> KIPEHLIGKGAEADIKRDSYLDFDVIIKERVKKGYRDERLDENIRKSRTAREARYLALVKDFGIPAPYIFDVDLDNKRIMMSYINGKLAKDVIEDNLDIAYKIGEIVGKLHKNDVIHNDLTTSNFIFDKDLYIIDFGLGKISNLDRDKAVDLIVFKKAVLSTHHEKFDEIWERFLEGYKSVYDRWEIILELMKDVERRARYVE;> MDPMIIRGIRGARINNEIFNLGLKFQILNADVVATKKHVLHAINQAKTKKPIAKSFWMEILVRASGQRQIHEAIKIIGAKDGNVCLICEDEETFRKIYELIGGEIDDSVLEINEDKERLIREIFKIRGFGNVVERVLEKIALIELKKE;> MDPMICLGLEGTAEKTGVGIVTSDGEVLFNKTIMYKPPKQGINPREAADHHAETFPKLIKEAFEVVDKNEIDLIAFSQGPGLGPSLRVTATVARTLSLTLKKPIIGVNHCIAHIEIGKLTTEAEDPLTLYVSGGNTQVIAYVSKKYRVFGETLDIAVGNCLDQFARYVNLPHPGGPYIEELARKGKKLVDLPYTVKGMDIAFSGLLTAAMRAYDAGERLEDICYSLQEYAFSMLTEITERALAH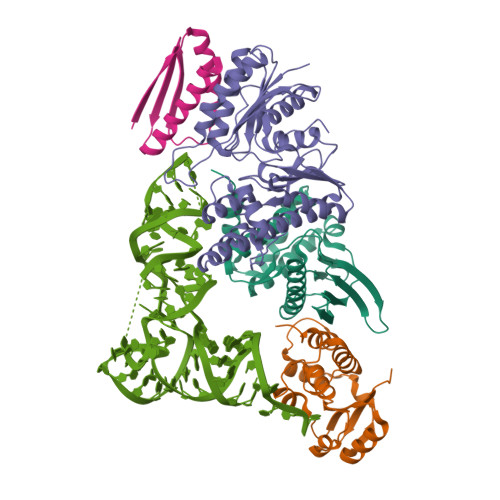TNKGEVMLVGGVAANNRLREMLKAMCEGQNVDFYVPPKEFCGDNGAMIAWLGLLMHKNGRWMSLDETKIIPNYRTDMVEVNWI;> MKAKRVQAKIEIEFPSEDVAKVVYEAVLYEHLSVPYRRSEIDFKLEGKKIILDIKATDSSALRGTVNSYLRWIKAAIDVIEV> GPTAAALEPHPEEKKKKRSGFRDRKVMEYENRIRAYSTPDKIFRYFATLKVISEPGEAEVFMTPEDFVRSITPNEKQPEHLGLDQYIIKRFDGKKISQEREKFADEGSIFYTLGECGLISFSDYIFLTTVLSTPQRNFEIAFKMFDLNGDGEVDMEEFEQVQSII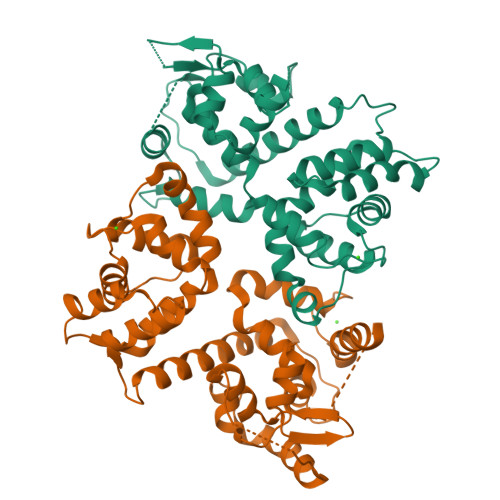RSQTSMGMRHRDRPTTGNTLKSGLCSALTTYFFGADLKGKLTIKNFLEFQRKLQHDVLKLEFERHDPVDGRITERQFGGMLLAYSGVQSKKLTAMQRQLKKHFKEGKGLTFQEVENFFTFLKNINDVDTALSFYHMAGASLDKVTMQQVARTVAKVELSDHVCDVVFALFDCDGNGELSNKEFVSIMKQRLMRGLEKPKDMGFTRLMQAMWKCAQETAWDFALPKQSNW;> HHSRVSVAARDGSFTVSAQKNVEHGIIYIGKPSLRKQRFMQFSSLEHEGEYYMTPRDFLFSVMFEQMERKTSVKKLTKKDIEDTLSGIQTAGCGSTFFRDLGDKGLISYTEYLFLLTILTKPHSGFHVAFKMLDTDGNEMIEKREFFKLQKIISKQDDLMTVKTNETGYQEAIVKEPEINTTLQMRFFGKRGQRKLHYKEFRRFMENLQTEIQEMEFLQFSKGLSFMRKEDFAEWLLFFTNTENKDIYWKNVREKLSAGESISLDEFKSFCHFTTHLEDFAIAMQMFSLAHRPVRLAEFKRAVKVATGQELSNNILDTVFKIFDLDGDECLSHEEFLGVLKNRMHRGLWVPQHQSIQEYWKCVKKESIKGVKEVWKQAGKGLF> ADPDPMKNTCKLLVVADHRFYRYMGRGEESTTTNYLIELIDRVDDIYRNTAWDNAGFKGYGIQIEQIRILKSPQEVKPGEKHYNMAKSYPNEEKDAWD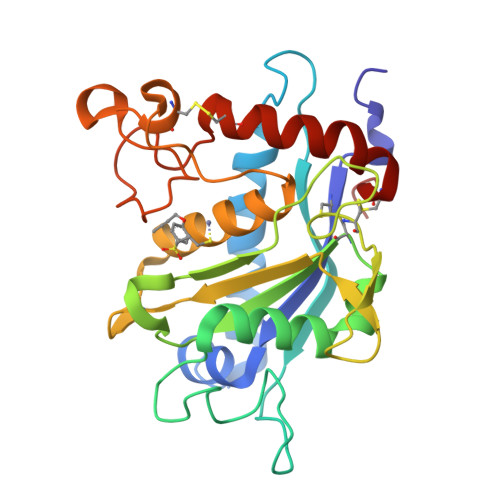VKMLLEQFSFDIAEEASKVCLAHLFTYQDFDMGTLGLAYVGSPRANSHGGVCPKAYYSPVGKKNIYLNSGLTSTKNYGKTILTKEADLVTTHELGHNFGAEHDPDGLAECAPNEDQGGKYVMYPIAVSGDHENNKMFSQCSKQSIYKTIESKAQECFQERS> MTGMSREEVESLIQEVLEVYPEKARKDRNKHLAVNDPAVTQSKKCIISNKKSQPGLMTIRGCAYAGSKGVVWGPIKDMIHISHGPVGCGQYSRAGRRNYYIGTTGVNAFVTMNFTSDFQEKDIVFGGDKKLAKLIDEVETLFPLNKGISVQSECPIGLIGDDIESVSKVKGAELSKTIVPVRCEGFRGVSQSLGHHIANDAVRDWVLGKRDEDTT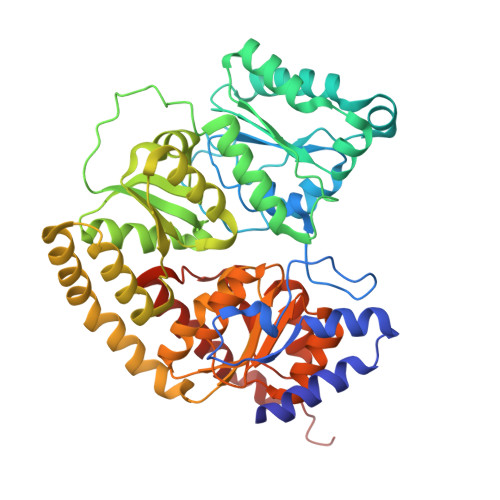FASTPYDVAIIGDYNIGGDAWSSRILLEEMGLRCVAQWSGDGSISEIELTPKVKLNLVHCYRSMNYISRHMEEKYGIPWMEYNFFGPTKTIESLRAIAAKFDESIQKKCEEVIAKYKPEWEAVVAKYRPRLEGKRVMLYIGGLRPRHVIGAYEDLGMEVVGTGYEFAHNDDYDRTMKEMGDSTLLYDDVTGYEFEEFVKRIKPDLIGSGIKEKFIFQKMGIPFREMHSWDYSGPYHGFDGFAIFARDMDMTLNNPCWKKLQAPWE> MHHHHHHHHHHGSVEDYKDDDDKGSMSEGVEAIVANDNGTDQVNGNRTGKDNEEHDGSTGSNLSNFLWHGGSVWDAWFSCASNQVAQVLLTLPYSFSQLGMLSGIVLQIFYGLLGSWTAYLISVLYVEYRARKEKEGKSFKNHVIQWFEVLDGLLG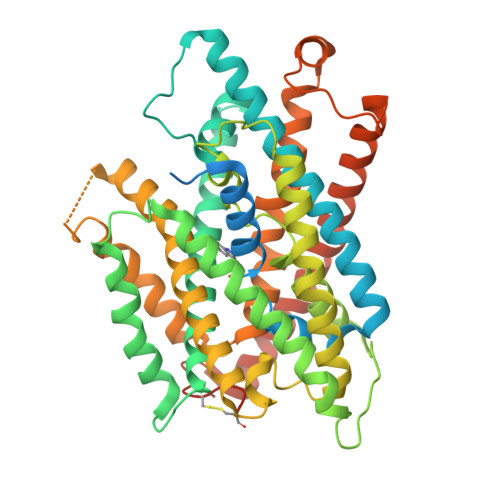SYWKALGLAFNCTFLLFGSVIQLIACASNIYYINDHLDKRTWTYIFGACCATTVFIPSFHNYRIWSFLGLGMTTYTAWYLAIASIIHGQAEGVKHSGPTKLVLYFTGATNILYTFGGHAVTVEIMHAMWKPQKFKYIYLMATLYVFTLTIPSAAAVYWAFGDALLDHSNAFSLMPKNAWRDAAVILMLIHQFITFGFACTPLYFVWEKVIGMHDTKSICLRALARLPVVIPIWFLAIIFPFFGPINSAVGALLVSFTVYIIPSLAHMLTYRSASARQNAAEKPPFFMPSWTAMYVLNAFVVVWVLIVGFGFGGWASVTNFVRQVDTFGLFAKCYQCKPAAAAAHAPVSALHHRL>VRKLRAEMEELKSMLSQL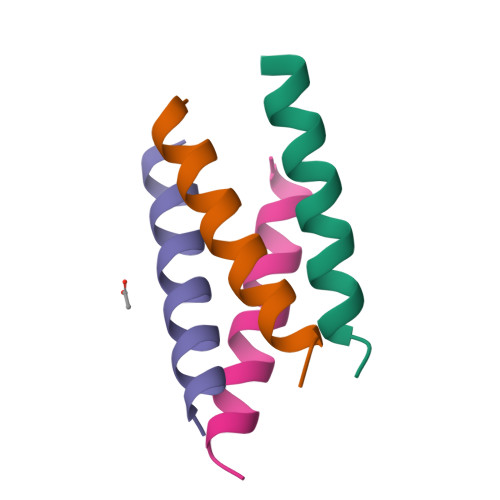GKT[8x]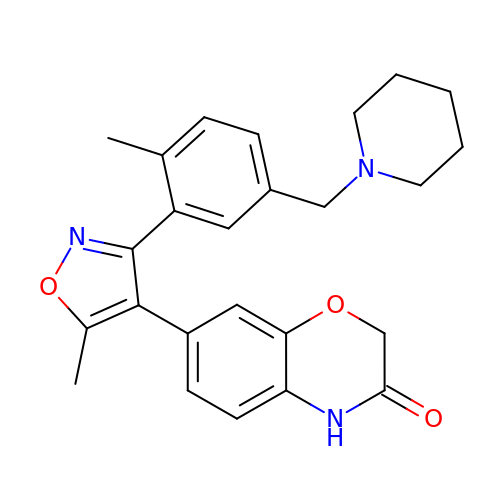7-[5-methyl-3-[2-methyl-5-(piperidin-1-ylmethyl)phenyl]-1,2-oxazol-4-yl]-4~{H}-1,4-benzoxazin-3-one | C25 H27 N3 O3 | GCVYFXYBQCKHCH-UHFFFAOYSA-N>UGGGGAGCCGAAAGGC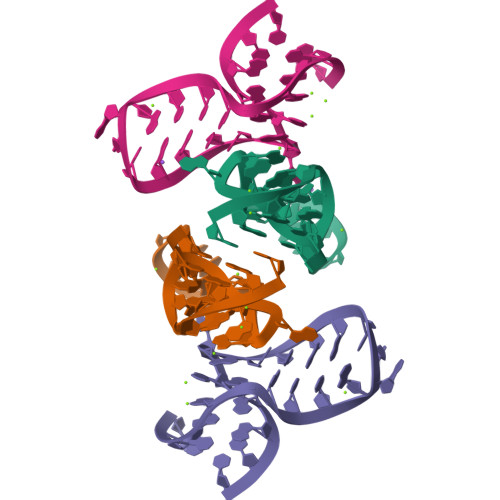GAAGAACC[8x]(2R,3R)-4-[4-(2-chlorophenyl)piperazin-1-yl]-2,3-dihydroxy-4-oxo-N-(2-thiophen-2-ylethyl)butanamide 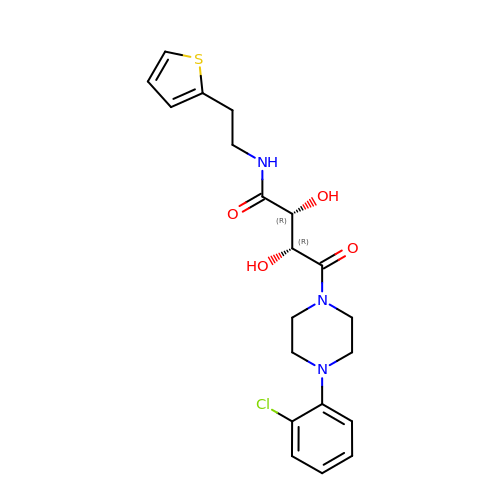| C20 H24 Cl N3 O4 S | AZEKZZSSVLIPCQ-QZTJIDSGSA-N> MNCIVCIEYIIVALMIISAILAVEWRDLLASTVGMAAVSLFASILFFFLQAPDVAMTEAAIGAALSAAVFIFAIK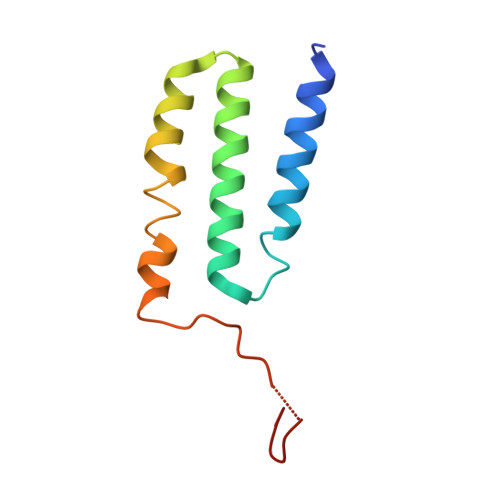RTYRYETEEEEKLGWWVRW Rv1625c is one of 16 adenylyl cyclases encoded in the genome of Mycobacterium tuberculosis. Adenylyl cyclases convert ATP to cyclic AMP, and these enzymes are classified into six types based on their sequence similarity. In solution Rv1625c exists predominantly as a monomer, with a small amount of dimer. It has been shown previously that the monomer is active and the dimeric fraction is inactive.

Rv1625c-Wt crystallized as a domain-swapped dimer. Two subunits (A and B) were obtained in the asymmetric unit with extensive domain swapping. Clear electron density is observed for residues 240–426 of chain A (except for the β1–α2, α3–β4 and β7–β8 loops) and for residues 240–428 of chain B (except for the β1–α2 and β7–β8 loops). In general small regions are involved in domain swapping, but in this case about half of the residues (β5–α4–β6–α5–β7–β8) are swapped between the subunits, leading to a large number of interactions between the subunits. The dimer has a head-to-head arrangement instead of the head-to-tail arrangement which is seen in the case of dimeric active ACs or GCs. The intact substrate-binding pockets at the active dimer interface are not formed in the swapped dimer. Metal ions and the substrate analogue cordycepin added during crystallization were not seen in the structure because of the altered domain arrangement that is not conducive for binding ligands. In the case of Rv1625c-Wt the dimerization-arm loop (β4–β5 loop) opened up and exchanges the part of the molecule consisting of the β5–α4–β6–α5–β7–β8 structural elements with the other subunit. Consequently, a new open interface is formed between the α2 helices of each subunit. A sulfate ion found in the new open interface neutralizes the positive charge present at the interface, interacting with the arginine side chains from both subunits.

>[2x]GAMEAEHDRSEALLANMLPASIAERLKEPERNIIADKYDEASVLFADIVGFTERASSTAPADLVRFLDRLYSAFDELVDQHGLEKIKVSGDSYMVVSGVPRPRPDHTQALADFALDMTNVAAQLKDPRGNPVPLRVGLATGPVVAGVVGSRRFFYDVWGDAVNVASRMESTDSVGQIQVPDEVYERLKDDFVLRERGHINVKGKGVMRTWYLIGRKVAADPGEVRGAEPRTAGV> GIVIPPKALFTQQGGAYGRCPNGTRALTVAELRGNAELQTYLRQITPGWSIYGLYDGTYLGQAYGGIIKDAPPGAGFIYRETFCITTIYKTGQPAADHYYSKVTATRLLASTNSRLCAVFVRDGQSVIGACASPYEGRYRDMYDALRRLLYMIYMSGLAVRVHVSKEEQYYDYE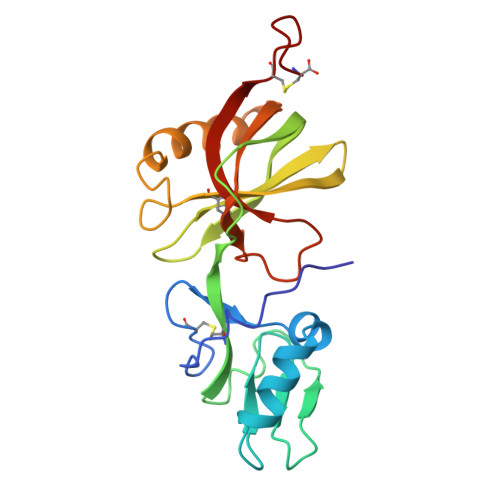DATFQTYALTGISLCNPAASIC>[6x]MHEPMKTLKNIHAEIRICQKFPKSTVQKRFSEFEELIKAASKNARNWKPISSVELFQGDSSLNELFEKLVIGTCELRDGELFENVNDLTINPSNIHVYKLHKDGPLSQNIGDDDGDESIIGSQLWQLPCVEFDSIWENLIYDSNLKNEVMSYVAALARLSEKHVNTKIINVNRLILLTGPPGTGKTSLCKGLAQHLSIRMNDK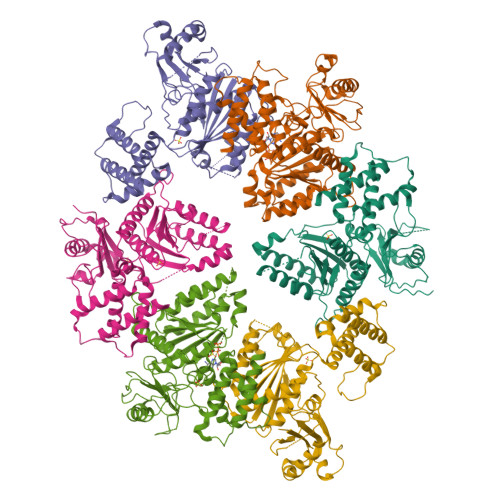YSKSVMLEINSHSLFSKWFSESGKLVQKMFDQIDELAEDEKCMVFVLIDEVESLGMCRESSSSRSEPSDAIRAVNALLTQIDRIRRRDNVLILCTSNLESTLDKALVDRADIVKNVGQPSDFARYSMLKSSIMELARIGVVIDNEVHTDYWPQDICDTKAPRNEFTEILFKIAQEARGLSGRAISMLPTLVYSKSPEETITLPNCMNLFLEAVKERLSRNN> DRLTVVKQYVDNVLNKASDTYHGDKPSPLLADGVDPRTGQQLEWIFPDGRRAVLSNFSAQQNLMRVMSGLSQLSGDPRYQKRAEDIVRYHFQNYQDPSGLLYWGGHRFVDLKTLQPEGPSEKEMVHELKNAYPYYDLMFSVDSDATARFIRGFWNAHVYDWRILETSRHGEYGKPMGALWESKFEQQPPFFATKGLSFLNAGNDLIYSASLLYKHQQDQGALTWAKRLADQYVLPRDAKTGLGVYQFTQALKREEPTDDADTHSKFGDRAQRQFGPEF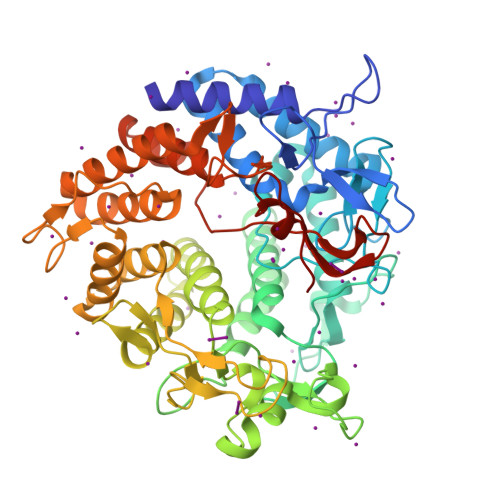GPTALEGNMMLKGRTSTLYSENALMQLQLGKDLGPQGQDLLKWTVDGLKAFAKYAYNDQDNTFRPMIANGQDLSNYTLPRDGYYGKKGTVLKPYKAGNEFLISYARAYAIDNDPLLWKVARGIANDQGLGDIGTAPGKEVKVNMDTTNSDPYALFALLDLYHASQVADYRKLAEKIGDNIIKIRYIDGFFMASSDRQYADVDAIEPYALLALEASLRNKPQAVAPFLNGAGFTEGAYRMDDGSARVSTRDNELFLLNVGEKLQPN>MTERPRDCRPVVRRARTSDVPAIKQLVDTYAGKILLEKNLVTLYEAVQEFWVAEHPDLYGKVVGCGALHVLWSDLGEIRTVAVDPAMTGHGIGHAIVDRLLQVARDLQLQRVFVLTFETEFFARHGFTEIEGTPVTAEVFDEMCRSYDIGVAEFLDLSYVKPNILGNSR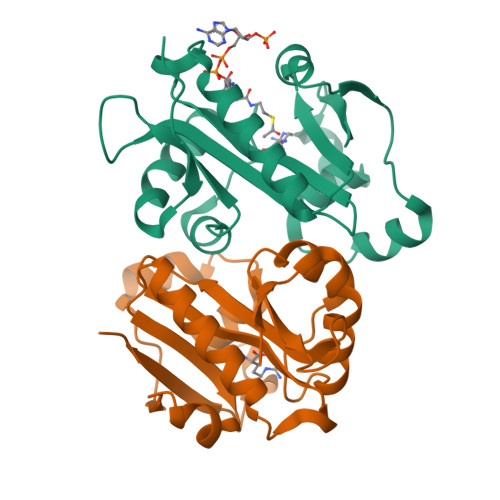MLLVLLEHHHHHH[2x]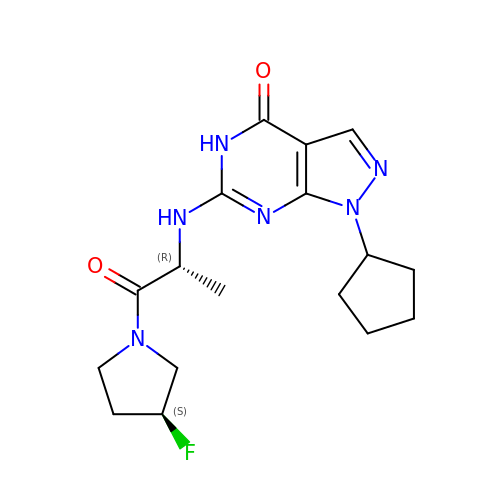1-cyclopentyl-6-({(2R)-1-[(3S)-3-fluoropyrrolidin-1-yl]-1-oxopropan-2-yl}amino)-1,5-dihydro-4H-pyrazolo[3,4-d]pyrimidin-4-one | C17 H23 F N6 O2 | HOQGZKUBNCAZBE-MNOVXSKESA-N> GIEDLITEVAQGALTLSLPKQQDSLPDTKASGPAHSKEVPALTAVETGATNPLVPSDTVQTRHVIQRRSRSESTIESFFARGACVAIIEVDNEEPTTRAQKLFAMWRITYK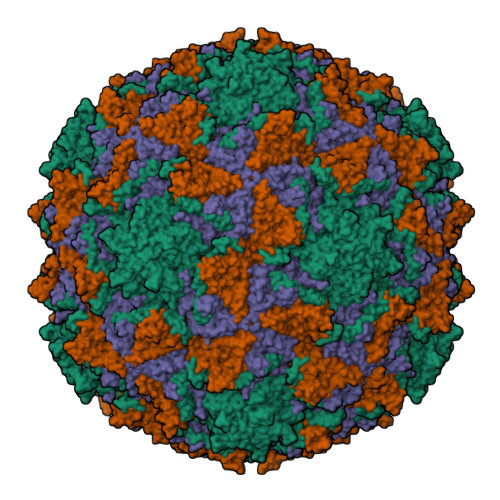DTVQLRRKLEFFTYSRFDMELTFVVTANFTNTNNGHALNQVYQIMYIPPGAPTPKSWDDYTWQTSSNPSIFYTYGAAPARISVPYVGLANAYSHFYDGFAKVPLKTDANDQIGDSLYSAMTVDDFGVLAIRVVNDHNPTKVTSKVRIYMKPKHVRVWCPRPPRAVPYYGPGVDYKDNLNPLSEKGLTTY;> SPNVEACGYSDRVLQLTIGNSTITTQEAANSVVAYGRWPEFIRDDEANPVDQPTEPDVATCRFYTLDTVMWGKESKGWWWKLPDALRDMGLFGQNMYYHYLGRSGYTVHVQCNASKFHQGALGVFAIPEYCLAGDSDKQRYTSYANANPGEKGGKFYSQFNRDTAVTSPKREFCPVDYLLGCGVLLGNAFVYPHQIINLRTNNSATIVLPYVNAMAIDSMVKHNNWGIAILPLSPLDFAQESSVEIPITVTIAPMCSEFNGLRNVTAPKFQ;> GLPVLNTPGSNQYLTSDNYQSPCAIPEFDVTPPIDIPGEVKNMMELAEIDTMIPLNLENTKRNTMDMYRVTLSDSADLSQPILCFSLSPASDPRLSHTMLGEVLNYYTHWAGSLKFTFLFCGSMMATGKILVAYAPPGAQPPTSRKEAMLGTHVIWDLGLQSSCTMVVPWISNVTYRQTTQDSFTEGGYISMFYQTRIVVPLSTPKSMSMLGFVSACNDFSVRLLRDTTHISQSALPQ;> MGAQVSSQKVGAHENSNRAYGGSTINYTTINYYKDSASNAASKQDYSQDPSKFTEPLKDVLIKTAPALN>GSAYLSELENRVKDLENKNSELEER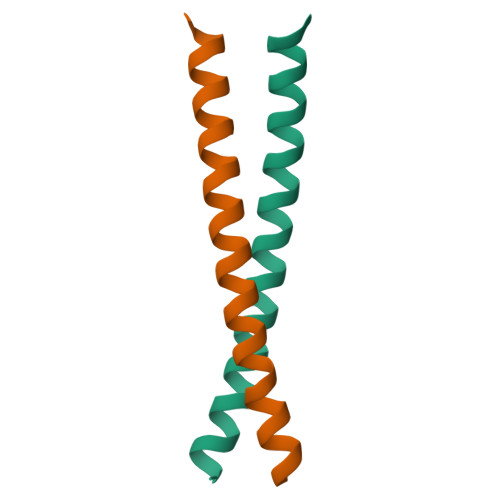LSTLQNENQMLRHILKN[2x]>[14x]MEQAMRERSELARKGIARAKSVVALAYAGGVLFVAENPSRSLQKISELYDRVGFAAAGKFNEFDNLRRGGIQFADTRGYAYDRRDVTGRQLANVYAQTLGTIFTEQAKPYEVELCVAEVAHYGETKRPELYRITYDGSIADEPHFVVMGGTTEPIANALKESYAENASLTDALRIAVAALRA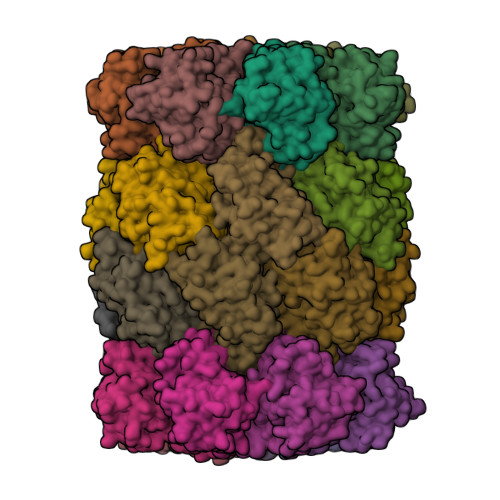GSADTSGGDQPTLGVASLEVAVLDANRPRRAFRRITGSALQALLVDQESPQSDGESSG;>TTIVALKYPGGVVMAGDRRSTQGNMISGRDVRKVYITDDYTATGIAGTAAVAVEFARLYAVELEHYEKLEGVPLTFAGKINRLAIMVRGNLAAAMQGLLALPLLAGYDIHASDPQSAGRIVSFDAAGGWNIEEEGYQAVGSGSLFAKSSMKKLYSQVTDGDSGLRVAVEALYDAADDDSATGGPDLVRGIFPTAVIIDADGAVDVPESRIAELARAIIESRSGADTFGSDGGEK[14x]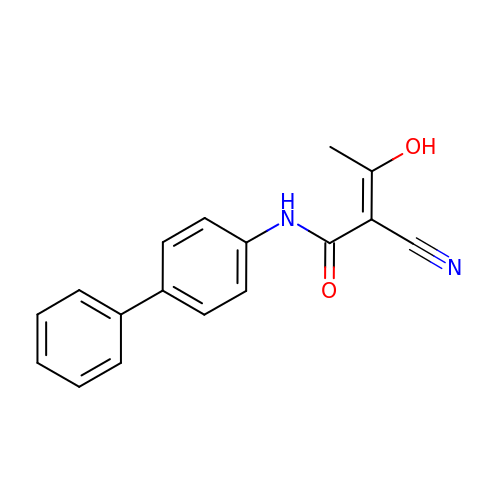(2Z)-N-biphenyl-4-yl-2-cyano-3-hydroxybut-2-enamide | C17 H14 N2 O2 | MUVPBAIVOHJDOC-VBKFSLOCSA-N> MKSVITTVISAADSAGRFPSSSDLESVQGNIQRASARLEAAEKLASNHEAVVKEAGDACFGKYGYLKNPGEAGENQEKINKCYR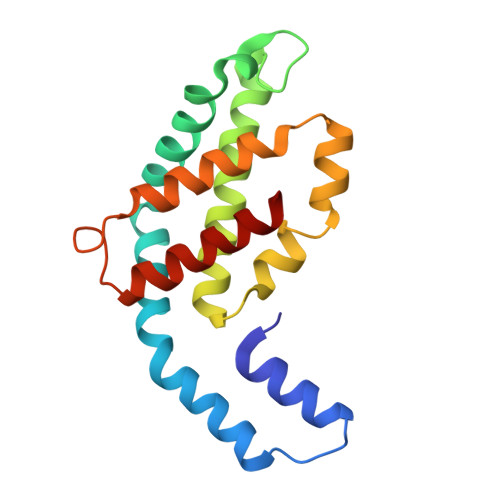DIDHYMRLVNYSLVIGGTGPLDEWGIAGAREVYRTLNLPTSAYIAAFAFTRDRLCGPRDMSAQAGVEYSTALDYIINSLS>[4x]SGAPEGAEYLRAVLRAPVYEAAQVTPLQKMEKLSSRLDNVILVKREDRQPVHSFKL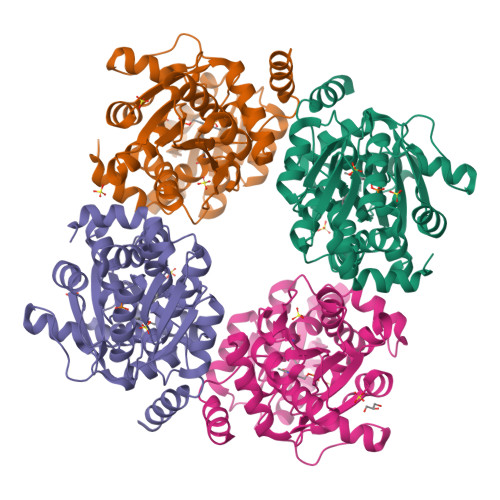RGAYAMMAGLTEEQKAHGVITASAGNHAQGVAFSSARLGVKALIVMPTATADIKVDAVRGFGGEVLLHGANFDEAKAKAIELSQQQGFTWVPPFDHPTVIAGQGTLALELLQQDAHLDRVFVPVGGGGLAAGVAVLIKQLMPQIKVIAVEAEDSACLKAALDAGHPVDLPRVGLFAEGVAVKRIGDETFRLCQEYLDDIITVDSDAICAAVKDLFEDVRAVAEPSGALALAGMKKYIAQHNIRGERLAHILSGANVNFLGLRYVLERCELLELE>MLNPIVRKFQYGQHTVTLETGMMARQATAAVMVSMDDTAVFVTVVGQKKAKPGQDFFPLTVNYQERTYAAGRIPGSFFRREGRPSEGETLIARLIDRPIRPLFPEGFVNEVQVIATVVSVNPQVNPDIVAMIGASAALSLSGIPFNGPIGAARVGYINDQYVLNPTQDELKESKLDLVVAGTEAAVLMVESEAQLLSEDQMLGAVVFGHEQQQVVIQNINELVKEAGKPRWDWQPEPVNEALNARVAALAEARLSDAYRITDKQERYAQVDVIKSETIATLLAEDETLDENELGEILHAIEKNVVRSRVLAGEPRIDGREKDMIRGLDVRTGVLPRTHGSALFTRGETQALVTATLGTARDAQVLDELMGERTDTFLFHYNFPPYSVGETGMVGSPKRREIGHGRLAKRGVLAVMPDMDKFPYTVRVVSEITESNGSSSMASVCGASLALMDAGVPIKAAVAGIAMGLVKEGDNYVVLSDILGDEDHLGDMDFKVAGSRDGISALQMDIKIEGITKEIMQVALNQAKGARLHILGVMEQAINAPRGDIS[12x];>[12x]EAPRHSDWQRPTFAFEGKGAAGGHTATHHASAAPARPQPVE

One widely occurring ribonuclease with such multi-functional versatility is polynucleotide phosphorylase, a phosphorolytic exoribonuclease (PNPase; polyribonucleotide nucleotidyltransferase; EC 2.7.7.8).5,6 PNPase processively cleaves single-stranded RNA substrates in the 3′-to-5′ direction using inorganic phosphate to attack the phosphoester linkage at the 3′ terminus and liberate nucleoside diphosphate. E. coli PNPase core forms a homotrimer with a ring-like architecture that encloses a large central channel. The two RNase PH-like domains within each protomer are spatially related by a pseudo-dyad axis, so that the PNPase trimer has approximate dihedral symmetry D3. In the current study, we solved several crystal structures of E. coli PNPase core bound to its cognate RNase E micro-domain, including a complex with O2′-methyl-modified RNA bound and another with manganese in the active site.

PNPase core was co-crystallised with its RNase E recognition micro-domain (residues 1021–1061) under four different conditions, providing several independent views of the micro-domain–enzyme interaction. The location of the micro-domain on the surface of PNPase is corroborated by an orthorhombic crystal form that, while diffracting to only limited resolution (roughly 3.6 Å), has four independent PNPase trimers in the asymmetric unit that reveal unbiased density for 12 copies of the RNase E micro-domain (results not shown). A segment of 20 amino acids from the RNase E C-terminal domain forms hydrogen-bonding interactions with the exposed ridge of the amino-terminal RNase PH domain of PNPase in an extended β-sheet and also makes van der Waals interactions through a small helical segment. The interaction is at a distance from the active site, and it does not affect enzyme activity (S. Nurmohamed et al., unpublished results).> MDEATWERMWKHVAKIHPDGEKVAQRIRGATDLPKIPIPSVPTFQPSTPVPERLEAVQRYIRELQYNHTGTQFFEIKKSRPLTGLMDLAKEMTKEALPIKSLEAVILGIYLTNSMPTLERFPISFKTYFSGNYFRHIVLGVNFAGRYGALGMSRREDLMYKPPAFRTLSELVLDFEAAYG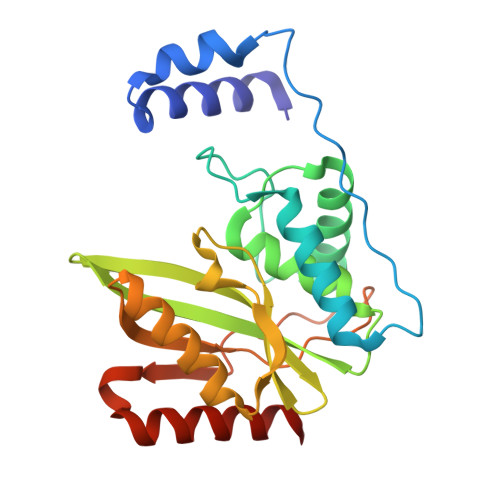RCWHVLKKVKLGQSVSHDPHSVEQIEWKHSVLDVERLGRDDFRKELERHARDMRLKIG> MPLCLKINKKHGEQTRRILIENNLLNKDYKITSEGNYLYLPIKDVDEDILK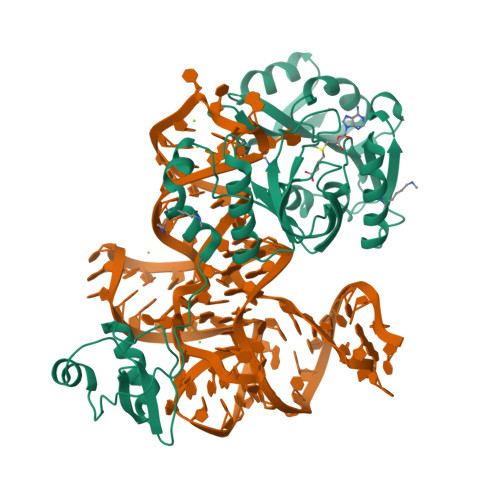SILNIEFELVDKELEEKKIIKKPSFREIISKKYRKEIDEGLISLSYDVVGDLVILQISDEVDEKIRKEIGELAYKLIPCKGVFRRKSEVKGEFRVRELEHLAGENRTLTIHKENGYRLWVDIAKVYFSPRLGGERARIMKKVSLNDVVVDMFAGVGPFSIACKNAKKIYAIDINPHAIELLKKNIKLNKLEHKIIPILSDVREVDVKGNRVIMNLPKFAHKFIDKALDIVEEGGVIHYYTIGKDFDKAIKLFEKKCDCEVLEKRIVKSYAPREYILALDFKINKK>[2x]MEQSRSQQRGGEQSWWGSDPQYQYMPFEHCTSYGLPSENGGLQHRLRKDAGPRHNVHPTQIYGHHKEQFSDREQDIGMPKKTGSSSTVDSKDEDHYSKCQDCIHRLGQVVRRKLGEDGIFLVLLGLLMALVSWSMDY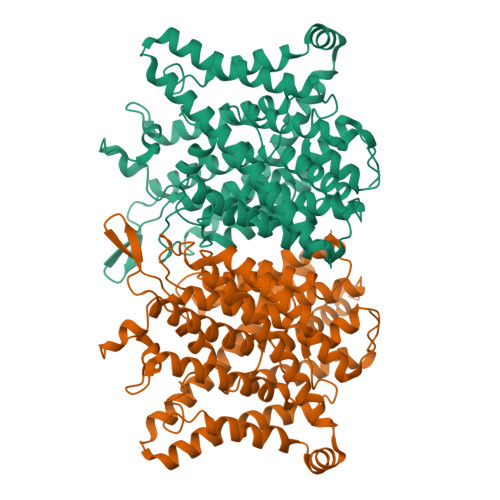VSAKSLQAYKWSYAQMQPSLPLQFLVWVTFPLVLILFSALFCHLISPQAVGSGIPEMKTILRGVVLKEYLTMKAFVAKVVALTAGLGSGIPVGKEGPFVHIASICAAVLSKFMSVFCGVYEQPYYYSDILTVGCAVGVGCCFGTPLGGVLFSIEVTSTYFAVRNYWRGFFAATFSAFVFRVLAVWNKDAVTITALFRTNFRMDFPFDLKELPAFAAIGICCGLLGAVFVYLHRQVMLGVRKHKALSQFLAKHRLLYPGIVTFVIASFTFPPGMGQFMAGELMPREAISTLFDNNTWVKHAGDPESLGQSAVWIHPRVNVVIIIFLFFVMKFWMSIVATTMPIPCGGFMPVFVLGAAFGRLVGEIMAMLFPDGILFDDIIYKILPGGYAVIGAAALTGAVSHTVSTAVICFELTGQIAHILPMMVAVILANMVAQSLQPSLYDSIIQVKKLPYLPDLGWNQLSKYTIFVEDIMVRDVKFVSASYTYGELRTLLQTTTVKTLPLVDSKDSMILLGSVERSELQALLQRHLCPERRLRAAQEMARKLSELPYDGKARLAGEGLPGAPPGRPESFAFVDEDEDEDLSGKSELPPSLALHPSTTAPLSPEEPNGPLPGHKQQPEAPEPAGQRPSIFQSLLHCLLGRARPTKKKTTQDSTDLVDNMSPEEIEAWEQEQLSQPVCFDSCCIDQSPFQLVEQTTLHKTHTLFSLLGLHLAYVTSMGKLRGVLALEELQKAIEGHTKSGVQLRPPLASFRNTTSTRKSTGAPPSSAENWNLPEDRPGATGTGDVIAASPETPVPSPSPEPPLSLAPGKVEGELEELELVESPGLEEELADILQGPSLRSTDEEDEDELIL>MTVVPENFVPGLDGVVAFTTEIAEPDKDGGALRYRGVDIEDLVSQRVTFGDVWALLVDGNFGSG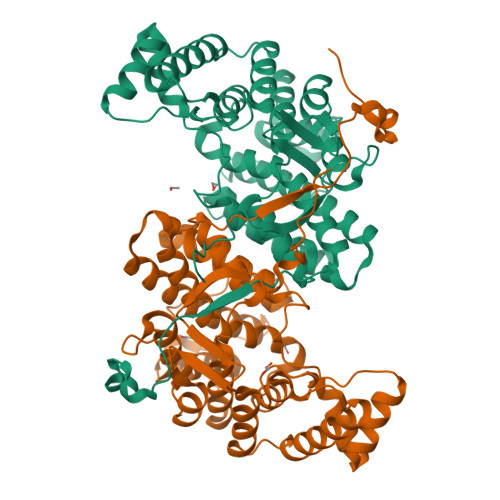LPPAEPFPLPIHSGDVRVDVQAGLAMLAPIWGYAPLLDIDDATARQQLARASVMALSYVAQSARGIYQPAVPQRIIDECSTVTARFMTRWQGEPDPRHIEAIDAYWVSAAEHGMNASTFTARVIASTGADVAAALSGAIGAMSGPLHGGAPARVLPMLDEVERAGDARSVVKGILDRGEKLMGFGHRVYRAEDPRARVLRAAAERLGAPRYEVAVAVEQAALSELRERRPDRAIETNVEFWAAVVLDFARVPANMMPAMFTCGRTAGWCAHILEQKRLGKLVRPSAIYVGPGPRSPESVDGWERVLTTAHHHHHH[4x]>MKAVQYTEIGSEPVVVDIPTPTPGPGEILLKVTAAGLCHSDIFVMDMPAAQYAGGLPLTLGHEGVGTVAELGEGVTGFGVGDAVAVYGPWGCGACHACARGRENYCTRAADLGITPPGYGSPGSMAEYMIVDSARHLVPIGDLDPVAAAPLTDAGLTPYHAISRVLPLLGPGSTAVVIGVGGLGHVGIQILRAVSAARVIAVDLDDDRLALAREVGADAAVKSGAGAADAIRELTGG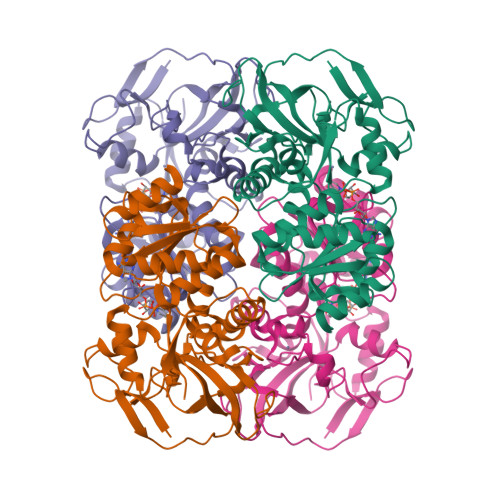QGATAVFDFVGAQSTIDTAQQVVAVDGHISVVGIHAGAHAKVGFFMIPFGASVVTPYWGTRSELMEVVALARAGRLDIHTETFTLDEGPAAYRRLREGSIRGRGVVVPTSHHHHH[4x]>NTVTEDTPATEQAVETPQPTAVSEEAPSSSKETKIPQTPGDAEETVADDANDLAPQAPAKTADTPATSKATIRDLNDPSQVKTLQEKAGKGAGTVVAVIDAGFDKNHEAWRLTDKTKARYQSKEDLEKAKKEHGITYGEWVNDKVAYYHDYSKDGKTAVDQEHGTHVSGILSGNAPSETKEPYRLEGAMPEAQLLLMRVEIVNGLADYARNYAQAIRDAVNLGAKVINMSFGNAALAYANLPDETKKAFDYAKSKGVSIVTSAGNDSSFGGKTRLPLADHPDYGVVGTPAAADSTLTVASYSPDKQLTETATVKTDDHQAKEMPVLSTNRFEPNKAYDYAYANRGMKEDDFKDVKGKIALIERGDIDFKDKIANAKKAGAVGVLIYDNQDKGFPIELPNVDQMPAAFISRKDGLLLKDNSKKTITFNATPKVLPTASDTKLSRFSSWGLTADGNIKPDIAAPGQDILSSVANNKYAKLSGTSMSAPLVAGIMGLLQKQYETQYPDMTPSERLDLAKKVLMSSATALYDEDEKAYFSPRQQGAGAVDAKKASAATMYVTDKDNTSSKVHLNNVSDKFEVTVTVHNKSDKPQELYYQATVQTDKVDGKHFALAPKALYETSWQKITIPANSSKQVTVPIDASRFSKDLLAQMKNGYFLEGFVRFKQDPKKEELMSIPYIGFRGDFGNLSALEKPIYDSKDGSSYYHEANSDAKDQLDGDGLQFYALKNNFTALTTESNPWTIIKAVKEGVENIEAIESSEITETIFAGTFAKQDDDSHYYIHRHANGKPYAAISPNGDGNRDYVQFQGTFLRNAKNLVAEVLDKEGNVVWTSEVTEQVVKNYNNDLASTLGSTRFEKTRWDGKDKDGKVVVNGTYTYRVRYTPISSGAKEQHTDFDVIVDNTTPEVATSATFSTEDRRLTLASKPKTSQPIYRERIAYTYMDEDLPTTEYISPNEDGTFTLPE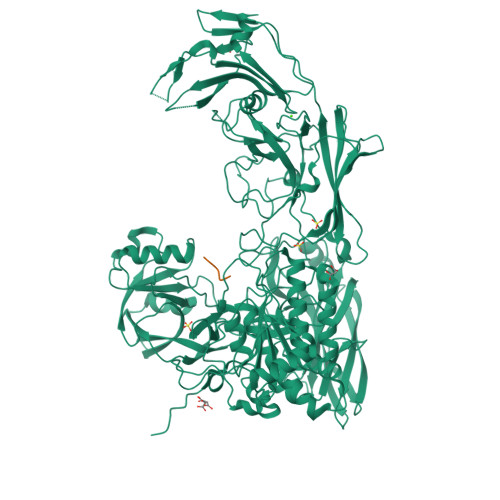EAETMEGGTVPLKMSDFTYVVEDMAGNITYTPVTKLLEGHS[2x]>[8x]MSTNKSEPTRKVDVHLTDNGTPFAYSMTSHKNVKVRAEVQPPLQLPGLIIFVHGVNSEGEWYDYAERSLCAGLNQRLGLEGEHGLKENNYEGGFFVNSDKSEGGWEHTYEIEGSQKKWVSGPRKITKGGDGRSPVIRFYWGYRAADNETDTYAIPLKNKKGDNYYDLPPESRKAKGPWFWGGGPFQNGCNQLVSLWSKTGFNNNPSLLGVPLPFSTQVLNGERDRLLSDAPPRHYYAHAAGRLAKLIKTIRNQHPEDTVTVLSHSQGTMIALAAAAIEAPDALFVMNSPYALENEPTTYISYPIKEIISRKARSATFADIVKKVAENKTRLKQQGCDNLLAGMSSDGNSWIPEGKTHNGLPERDNHGTTWIYCNPHDRVM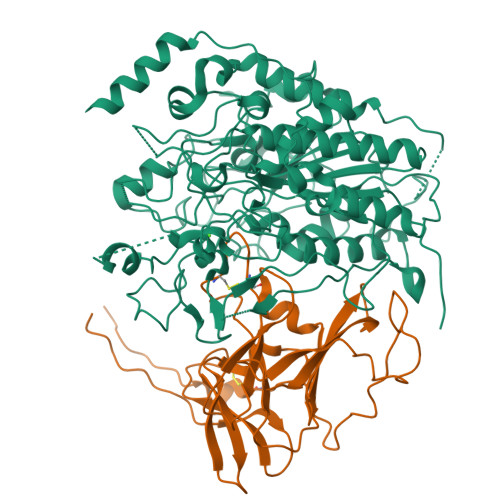GSSPLRSIGWQGLPDTKDGTPHTLFKQAGDTLYVRILGRNTPCGGTPTAQTHFSNLGDGKPFWDSTTTLLQRATWPDPDSGQTLTINAPQVPEPLTAEELKNFDQDYARDEKQSGGAGYAYGQINPETKKPVDTDYRYYISLYGYFDRKMVPKKDSGYYQSGPGSKEDRVKYEKQSQEEMLEEVRTYVQRPTDHSTLPSDERFMSRVVAYDLPIGYCWHSWDKAGLEELRRQADWLESDDYYFSGKLTVPPIPPAIKQDVAEDAEQRKAEEKARLRNV;>[8x]MLKEWMIFTCSLLTLAGASLPLSGCISRGQESISEGAAFGAGILREPGATKKADTKDLNVPPPVYGPPQVIFRIDDNRYFTLENYTHCENGQTFYNNKAKNIHVKILDASGYLFKGRLFWLSTRDDFLAFPATLNTRHASCMGSNKGCMNAVIVTTDGGKRRSGVPYGSYTQNPTGATRDYDMLVMNDGFYLLRYRGGQGRFSPVILRWILSTEDSSGVVRSEDAYELFRPGEEVPSTGFYKIDLSRFYPKNNVMEMQCDRTLEPVQPSESKIQ> GAMAGQGDGSVIELGEQTVVATAQEETKQAPGVSIITAEDIAKRPPSNDLSQIIRTMPGVNLTGNSSSGQRGNNRQIDIRGMGPENTLILVDGKPVSSRNSVRYGWRGERDSRGDTNWVPADQVERIEVIRGPAAARYGNGAAGGVVNIITKQAGAETHGNLSVYSNFPQHKAEGASERMSFGLNGPLTENLSYRVYGNIAKTDSDDWDINAGHESNRTGKQAGTLPAGREGVRNKDIDGLLSWRLTPEQTLEFEAGFSRQGNIYTGDTQNTNSNNYVKQMLGHETNRMYRETYSVTHRGEWDFGSSLAYLQYEKTRNSRINEGLAGGTEGIFDPNNAGFYTATLRDLTAHGEVNLPLHLGYEQTLTLGSEWTEQKLDDPSSNTQNTEEGGSIPGLAGKNRSSSSSARIFSLFAEDNIELMPGTMLTPGLRWDHHDIVGDNWSPSLNLSHALTERVTLKAGIARAYKAPNLYQLNPDYLLYSAGAGCYGQSTSCYLRGNDGLKAETSVNKELGIEYSHDGLVAGLTYFRNDYKNKIESGLSPVDHASGGKGDYANAAIYQWENVPKAVVEGLEGTLTLPLADGLKWSNNLTYMLQSKNKETGDVLSVTPRYTLNSML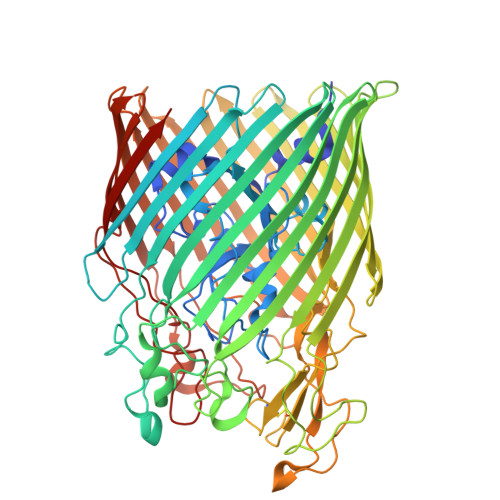DWQATDDLSLQATVTWYGKQKPKKYDYHGDRVTGSANDQLSPYAIAGLGGTYRLSKNLSLGAGVDNLFDKRLFRAGNAQGVVGIDGAGAATYNEPGRTFYTSLTASF> HHHHHHHHSQAGDTLNDVIQDPTRRNKLINDNNLLKGIIMGRDGPVPSSRELIVRPDTLRAIINNRATIETTTMEAEFTETLMESNYNSASVKVSAPCITANSEYSESSSFKNTETEKSMYTSSRCLFPQGRIDFTTPDSGFDDVIKLSPQFTSGVQAALAKATGTEKREALQNLFQEYGCVFRTKVHIGGVLSAHTMETFSRSENETEVKQDVKAGLEGAVKGWCGGATAGHGNTQGTITTSQNRKLNVKYIVNGGDYTKIQNTEEWVASTNQ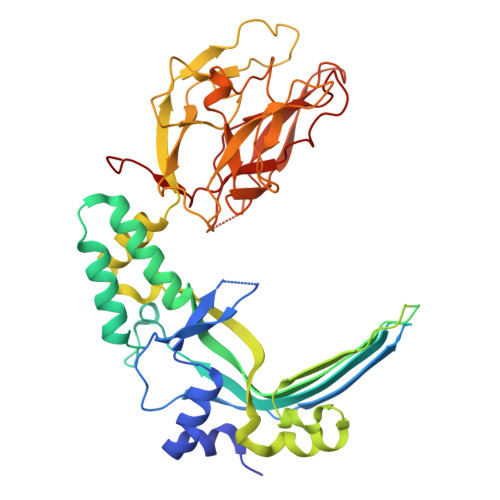SEHWRVIEVTEVTAVADLLPQPIRGQVKDLLKPLLGKWVDVEKVPGLESLPVSVYRPKGAIPAGWFWLGDTADASKALLVKPTLPARSGRNPALTSLHQGSGMTEQPFVDLPQYQYLSTYFGSFAHDTPPGSTLRGLRPDHVLPGRYEMHGDTISTAVYVTRPVDVPFPEDECFDLKSLVRVKLPGSGNPPKPRSALKKSMVLFDSGEK>[6x]FDASNFKDFSSIASASSSWQNQSGSTMIIQVDSFGNVSGQYVNRAQGTGCQNSPYPLTGRVNGTFIAFS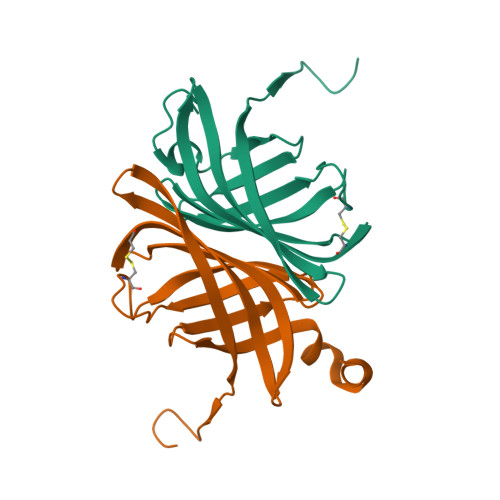VGWNNSTENCNSATGWTGYAQVNGNNTEIVTSWNLAYEGGSGPAIEQGQDTFQYVPTTENKSLLKD>[2x]NEDICFIAGIGDTNGYGWGIAKELSKRNVKIIFGIWPPVYNIFMKNYKNGKFDNDMIIDKDKKMNILDMLPFDASFDTANDIDEETKNNKRYNMLQNYTIEDVANLIHQKYGKINMLVHSLANAKEVQKDLLNTSRKGYLDALSKSSYSLISLCKYFVNIMKPQSSIISLTYHASQKVVPGYGGGMSSAKAALESDTRVLAYHLGRNYNIRINTISAGPLKSRAATAIN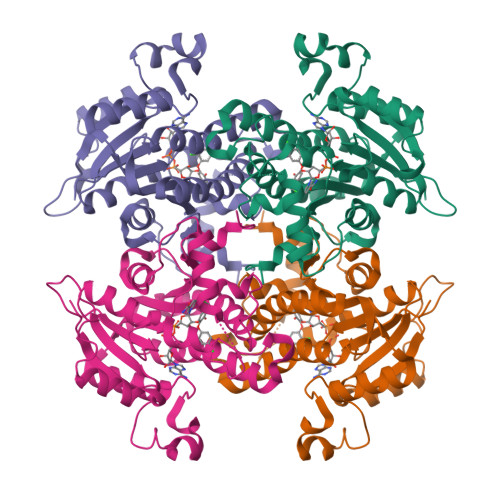KLNNTYENNTNQNKNRNRHDVHNIMNNSGEKEEKKISASQNYTFIDYAIEYSEKYAPLRQKLLSTDIGSVASFLLSRESRAITGQTIYVDNGLNIMFLPD> RRVIG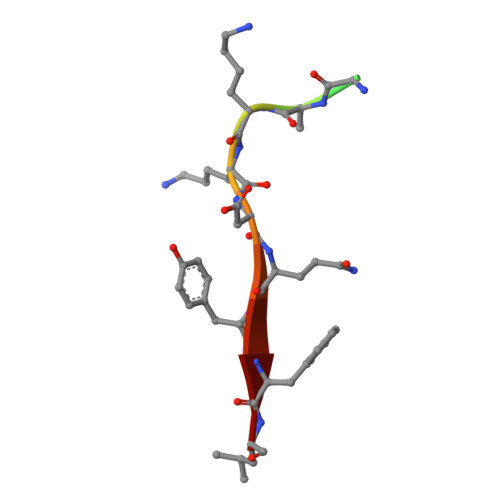AKKDQYFL>KSYKSVALVVGVTGIVGSSLAEVLKLPDTPGGPWKVYGVARRPCPVWLAKKPVEYIQCDVSDNQETISKLSPLKDITHIFYVSWIGSEDCQTNATMFKNILNSVIPNASNLQHVCLQTGIKHYFGIFEEGSKVVPHDSPFTEDLPRLNVPNFYHDLEDILYEETGKNNLTWSVHRPALVFGFSPCSMMNIVSTLCVYATICKHENKALVYPGSKNSWNCYADAVDADLVAEHEIWAAVDPKAKNQVLN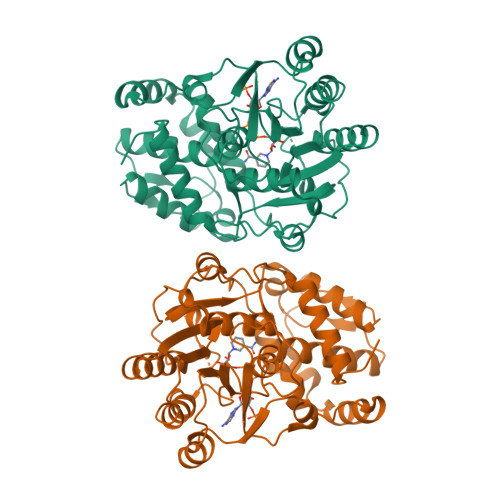CNNGDVFKWKHIWKKLAEEFGIEMVGYVEGKEQVSLAELMKDKDQVWDEIVKKNNLVPTKLKEIAAFWFADIAFCSENLISSMNKSKELGFLGFRNSMKSFVSCIDKMRDYRFIPASAWSHPQFEK[2x]>GIDPFTMSLQEPVSPVEESPTSTADRIADLAARHEEAVVLAEKKAADRQHLKGKLTARARIDLLLDPGSFVELDEFVRHRTVEAGIPRPYGDGVVTGHGTIDGRQVCVFSHDFTTLGGSMGEAFGSKVVKIYDFAMSVGCPVIGINDSGGARIQEGVMSIAYYTELGVRNVHSSGVIPQISLIMGPCAGGSVYSPALTDFTVMVKDISYMFVTGPEVVSAVMGEQVTAEQLGGPAVHAEVSGNAHYVGDDEQDAISWVQTLLGYLPPNNLDPAPVYDHDCAPGITEADLALDTVIPDSEQQVYDMADVITAVLDDGDYLEIHPDFARNIICALGRVEGHSVAVVANQPRHLAGVLDIDASEKAARFIRFCDSFNIPVLTFMDVPGYLPGVGQEHQGIIRRGIKLFYAYAESTVPKITVITRKAYGGGYAVMGSRQIGADRVMAWPTAEIAVMGANSAVPILHRRELAAVPPEERAAVKENLVDDYRRRFGNPYEAAAHGYVDMVISPSRTRYEVARALASLRNKRQARPARKHGNIPL[6x]

X-ray crystal structures of SamR0483 alone and in complex with hexanoyl-CoA reveal the molecular basis for medium chain acyl-CoA recognition by this unusual YCC β-subunit, prompting us to rename it medium chain acyl-CoA carboxylase beta subunit (MccB). Similar to other bacterial YCC β-subunits, MccB has 3–2 symmetry and is composed of three individual dimers that form a ring-like hexamer. Each monomer can be divided into two domains harbouring two copies of the crotonase fold that pack together in an antiparallel manner to form a dimer. Taken together, these results establish the existence of a unique YCC-dependent pathway for unusual polyketide extender unit biosynthesis.

To address this question structures of MccB bound to either one or four molecules of hexanoyl-CoA were solved to 2.75 and 2.85 Å, respectively. These co-crystal structures were obtained via incubation of MccB with 5 or 10 mM hexanoyl-CoA before crystallization. Interestingly, the electron density corresponding to residues 452–477 of monomer F was only present in the crystal form bound to four molecules of hexanoyl-CoA, suggesting that the helix-loop-helix lid region of MccB is stabilized at higher substrate concentrations. The first region is located at the entrance of the substrate binding pocket, which is characterized by a network of hydrogen bonds between the adenosine moiety of hexanoyl-CoA and the protein. The adenosine moiety is further stabilized by a hydrogen bond from the backbone carbonyl group of Pro453 to the 2' hydroxyl group of ribose. The structures of MccB with hexanoyl-CoA bound were compared with the previously-reported structure of PccB bound to propionyl-CoA 21. In the PccB co-crystal structure, propionyl-CoA binds close to the entrance of the active site, leaving the 3' phosphate of CoA more exposed to the solvent. In contrast, MccB sequesters its substrate deep into the active site via hydrophobic interactions between the side chains of the residues lining the substrate binding pocket and the aliphatic portion of hexanoyl-CoA. Further, the adenine ring of hexanoyl-CoA is tilted ∼90° with respect to that of the adenine-ring of propionyl-CoA in the PccB co-crystal structure. Superimposition of the substrate bound MccB and PccB structures strongly suggested that replacing Gly161 with Phe in MccB would cause a steric clash with the aliphatic chain of hexanoyl-CoA.> MTAQTTHTVDAVVIGAGFGGIYAVHKLHHELGLTTVGFDKADGPGGTWYWNRYPGALSDTESHLYRFSFDRDLLQESTWKTTYITQPEILEYLEDVVDRFDLRRHFKFGTEVTSALYLDDENLWEVTTDHGEVYRAKYVVNAVGLLSAINFPNLPGLDTFEGETIHTAAWPEGKSLAGRRVGVIGTGSTGQQVITSLAPEVEHLT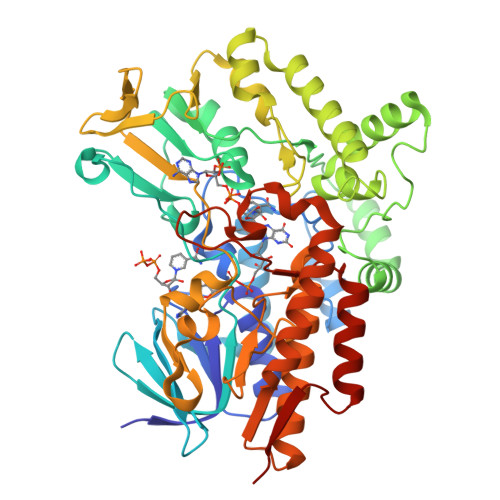VFVRTPQYSVPVGNRPVNPEQIAEIKADYDRIWERAKNSAVAFGFEESTLPAMSVSEEERNRIFQEAWDHGGGFRFMFGTFGDIATDEAANEAAASFIRAKVAEIIEDPETARKLMPKGLFAKRPLCDSGYYEVYNRPNVEAVAIKENPIREVTAKGVVTEDGVLHELDVLVFATGFDAVDGNYRRIEIRGRDGLHINDHWDGQPTSYLGVSTANFPNWFMVLGPNGPFTNLPPSIETQVEWISDTIGYAERNGVRAIEPTPEAEAEWTETCTEIANATLFTKGDSWIFGANIPGKKPSVLFYLGGLRNYRAVMAEVAADGYRGFEVKSAEMVTV>MKVSLAGQTVDVKKILNEIPKRTVTAALLEGGEIVAVEEADDEHAERKLVRRHDVEGKVVFVTARPCLYCARELAEAGVAGVVYLGRGRGLGPYYLARSGVEVVEVHPDEPLGYDPVDRLDVLLTFGGNPYLTEEDVAARVYCLLTGRGFDADIAPAPENLSGRVEIMVTRGDPDEAVELLKEELPVFRIRRFLISGEFDRDELRERILEDIEPRILDPFAVRARIARAGAFSSSREAEVFIGDVLTSVGREVNLNDPRTVVTVDVL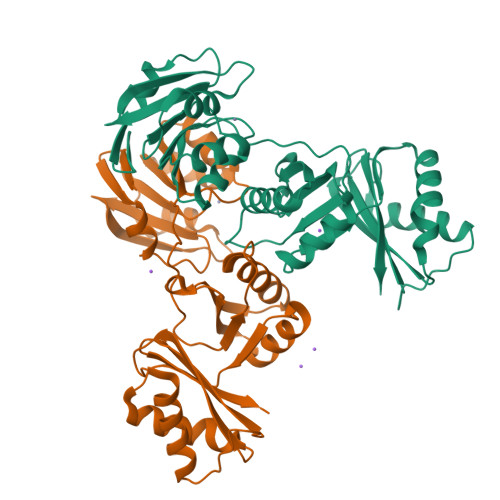GPRVSVGVEKR[4x]> MNRNVYAVLSTVLAASLLAACNSGGEQVKAESKNKTAATQQSEPNVIAAHKGVNQAPVPLKMERVGPHDVHIEMTAQITDIEIDKGKIYKAWTFNGQAPGPLVVVNEGDTIHFTLKNMDPVVPHSMDFHAVHASPSKDFIDVMPNKSGTFTYPANKPGVFMYHCGTKPVLQHIANGMHGVIIVKPKNGYPTDKEVDREYVLIQNEWYKYNDMNDFQNGVPSYVVFSSKALKPGDPNTNGDTFTLKEKPLLAKVGEKIRLYINNVGPNEVSSFHVVGTVFDDVYLDGNPNNHLQGMQTVMLPASGGA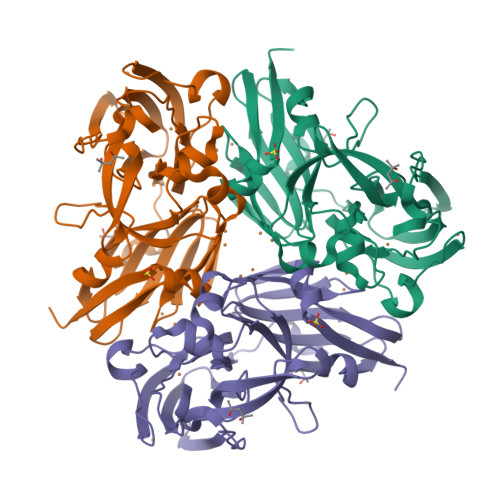VVEFTVTRPGTYPIVTHQFNHAQKGAVAMLKVTETGEDDGTETSGH> MQFLNMFFFDIYPYI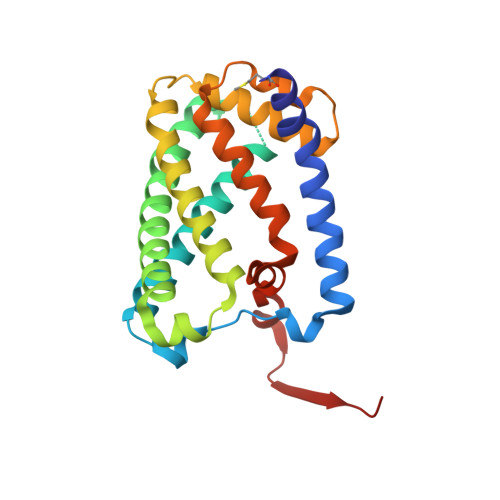AGAVFLIGSWLRYDYGQYTWRAASSQMLDRKGMNLASNLFHIGILGIFVGHFFGMLTPHWMYEAWLPIEVKQKMAMFAGGASGVLCLIGGVLLLKRRLFSPRVRATTTGADILILSLLVIQCALGLLTIPFSAQHMDGSEMMKLVGWAQSVVTFHGGASQHLDGVAFIFRLHLVLGMTLFLLFPFSRLIHIWSVPVEYLTRKYQLVRARH>[18x]M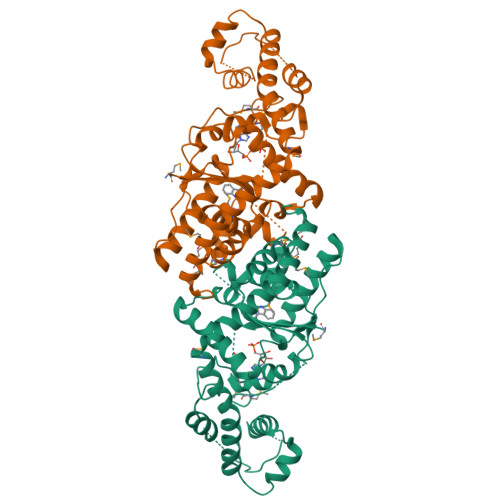KTIFSGIQPSGVITIGNYIGALRQFVELQHEYNCYFCIVDQHAITVWQDPHELRQNIRRLAALYLAVGIDPTQATLFIQSEVPAHAQAAWMLQCIVYIGELERMTQFKEKSAGKEAVSAGLLTYPPLMAADILLYNTDIVPVGEDQKQHIELTRDLAERFNKRYGELFTIPEARIPKVGARIMSLVDPTKKMSKSDPNPKAYITLLDDAKTIEKKIKSAVTDSEGTIRYDKEAKPGISNLLNIYSTLSGQSIEELERQYEGKGYGVFKADLAQVVIETLRPIQERYHHWMESEELDRVLDEGAEKANRVASEMVRKMEQAMGLGR> PNSMKNIESLFDYSAGQFEFIDHLLTMGVGVHFAALIFFLVVSQFVAPKYRIATALSCIVMVSAGLILNSQAVMWTDAYAYVDGSYQLQDLTFSNGYRYVNWMANIPCLLLQLLIVLNLKGKELFSTATWLILAAWGMIITGYVGQLYEVDDIAQL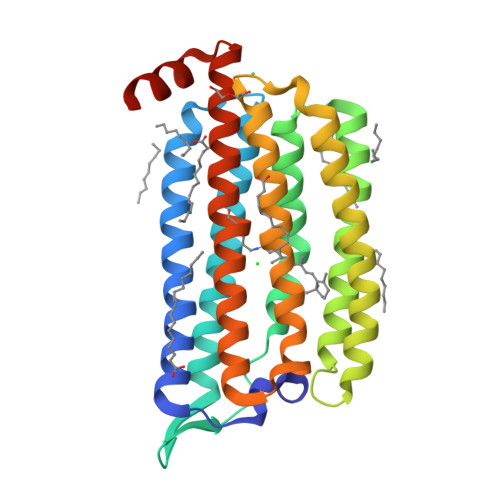MIWGAVSTAFFVVMNWIVGTKIFKNRATMLGGTDSTITKVFWLMMFAWTLYPIAYLVPAFMNNADGVVLRQLLFTIADISSKVIYGLMITYIAIQQSAAAGYVPAQQALGRIGMDSKAA> MRHISPEELIALHDANISRYGGLPGMSDPGRAEAIIGRVQARVAYEEITDLFEVSATYLVATARGHIFND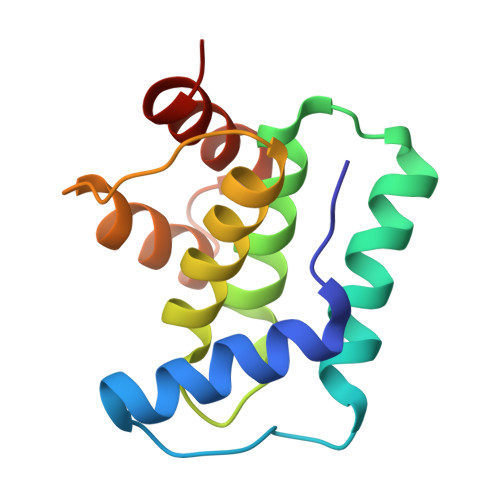ANKRTALNSALLFLRRNGVQVFDSPELADLTVGAATGEISVSSVADTLRRLYGSAE>NTSLEAIVQNASSDNQGIQLSAVQAARKLLSSDRNPPIDDLIKSGILPILVHCLERDDNPSLQFEAAWALTNIASGTSEQTQAVVQSNAVPLFLRLLHSPHQNVCEQAVWALGNIIGDGPQCRDYVISLGVVKPLLSFISPSIPITFLRNVTWVMVNLCRHKDPPPPMETIQEILPALCVLIHHTDVNILVDTVWALSYLTDAGNEQIQMVIDSGIVPHLVPLLSHQEVKVQTAALRAVGNIVTGTDEQTQVVLNCDALSHFPALLTHPKEKINKEAVWFLSNITAGNQQQVQAVIDANLVPMIIHLLDKGDFGTQKEAAWAISNLTISGRKDQVAYLIQQNVIPPFCNLLTVKDAQVVQVVLDGLSNILKMAEDEAETIGNLIEECGGLEKIEQLQNHENEDIYKLAYEIIDQFF[2x];>SGKRKLITSEEERSPAKRGRKS[2x]

53BP1 (TP53-binding protein 1), a key player in DNA double-strand break repair, has a classical bipartite nuclear localization signal (NLS) of sequence 1666-GKRKLITSEEERSPAKRGRKS-1686 that binds to importin-α, a nuclear import adaptor protein. Nucleoporin Nup153 is involved in nuclear import of 53BP1, and the binding of Nup153 to importin-α has been proposed to promote efficient import of classical NLS-containing proteins. Previous studies have shown that Nup153 is involved in nuclear import of 53BP1 and that the interaction between Nup153 and importin-α is required for efficient nuclear import of classical NLS-containing proteins. It has been proposed that the extreme C-terminus of Nup153 binds directly to importin-α.

Here, the ARM-repeat domain of human importin-α3 bound to 53BP1 NLS was crystallized in the presence of a synthetic peptide corresponding to the extreme C-terminus of Nup153 (sequence: 1459-GTSFSGRKIKTAVRRRK-1475). The crystal diffracted X-rays to 1.9 Å resolution, and the structure was solved by molecular replacement. The asymmetric unit contained two molecules of importin-α3 and two molecules of 53BP1 NLS. Although no convincing density was observed for the Nup153 peptide, the electron density corresponding to 53BP1 NLS was unambiguous and continuous along the entire length of the bipartite NLS. The structure revealed a novel dimer of importin-α3, in which two protomers of importin-α3 are bridged by the bipartite NLS of 53BP1. In this structure, the upstream basic cluster of the NLS is bound to the minor NLS-binding site of one protomer of importin-α3, whereas the downstream basic cluster of the same chain of NLS is bound to the major NLS-binding site of another protomer of importin-α3. However, no convincing density was observed for the Nup153C peptide. This quaternary structure of importin-α3–53BP1 NLS complex is distinctly different from the previously reported crystal structure of mouse importin-α1–53BP1 NLS complex, in which one molecule of 53BP1 NLS is bound along the concave surface of one molecule of importin-α1. • Although the quaternary structure reported here could be an artifact of the crystallization process, the data enriches structural database of what can happen during crystallization of protein-peptide complexes, and will benefit researchers interested in protein crystallization.>GPDSMKETLQPEHEKQIKVLQEELQTIEYKSCEICDNDIEKFLELMLAYKEATVNLMQEMVKSPSILHILKEGRL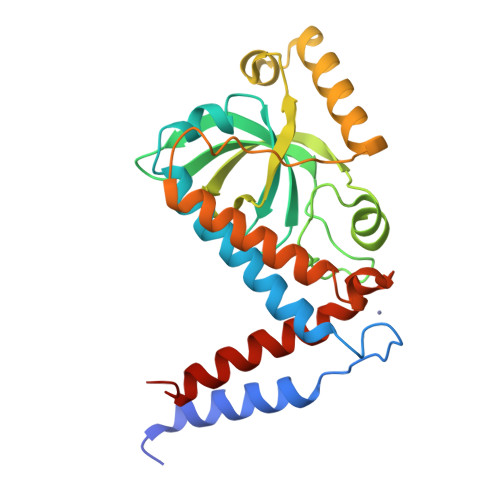VAFRDPNDCLKLGFVFKVSLKDAVCVIMTFTKPYKLPNGEPNHLIYFPKADGYRRRNFPKFQKTDFYMEEVPVTAIEVITKRKFAAPLGKVIKKDVAALNEFNAETNNILDGKTLKEAINIEKQGLKIHQILLDRTNIRDEIFKLKSIKCPNLSQHIVPKFKAHVIKKKIEELYHLMSDQN[5x]> PKDTIYHAKDAVQAT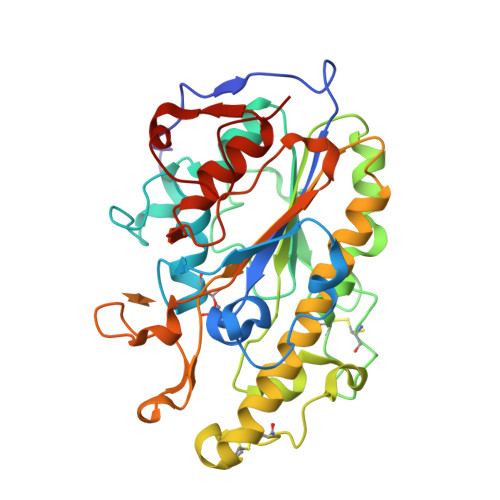KPDMRKPRLVVFVVGETARADHVSFNGYERDTFPQLAKIDGVTNFSNVTSCGTSTAYSVPCMFSYLGADEYDVDTAKYQENVLDTLDRLGVSILWRDNNSDSKGVMDKLPKAQFADYKSATNNAICNTNPYNECRDVGMLVGLDDFVAANNGKDMLIMLHQMGNHGPAYFKRYDEKFAKFTPVCEGNELAKCEHQSLINAYDNALLATDDFIAQSIQWLQTHSNAYDVSMLYVSDHGESLGENGVYLHGMPNAFAPKEQRSVPAFFWTDKQTGITPMATDTVLTHDAITPTLLKLFDVTADKVKDRTAFIRLEHHH>MSDMNNPSDENTGALDDLWADALNEQKATTTKSAADAVFQQLGGGDVSGAMQDIDLIMDIPVKLTVELGRTRMTIKELLRLTQGSVVALDGLAGEPLDILINGYLIAQGEVVVVADKYGVRITDIITPSERMRRLSR[9x];>[3x]MSATASTATQPKPLEWLNRLRANPRIPLIVAGSAAVAIVVAMVLWAKTPDYRTLFSNLSDQDGGAIVAQLTQMNIPYRFANGSGAIEVPADKVHELRLRLAQQGLPKGGAVGFELLDQEKFGISQFSEQVNYQRALEGELARTIETLGPVKSARVHLAMPKPSLFVREQKSPSASVTVTLEPGRALDEGQISAVVHLVSSAVAGLPPGNVTLVDQSGHLLTQSNTSGRDLNDAQLKFANDVESRIQRRIEAILSPIVGNGNVHAQVTAQLDFANKEQTEEHYSPNGDASKATLRSRQLNISEQVGAGYPGGVPGALSNQPAPPNEAPIATPPTNQQNAQNTPQTSTSTNSNSAGPRSTQRNETSNYEVDRTIRHTKMNVGDIERLSVAVVVNYKTLADGKPLPLTADQMKQIEDLTREAMGFSDKRGDTLNVVNSPFSAVDNTGGELPFWQQQSFIDQLLAAGRWLLVLVVAWILWRKAVRPQLTRRVEEAKAAQEQAQVRQETEEAVEVRLSKDEQLQQRRANQRLGAEVMSQRIREMSDNDPRVVALVIRQWMSNDHE;>MGDSILSQAEIDALLNGDSDTKDEPTPGIASDSDIRPYDPNTQRRVVRERLQALEIINERFARQFRMGLFNLLRRSPDITVGAIRIQPYHEFARNLPVPTNLNLIHLKPLRGTGLVVFSPSLVFIAVDNLFGGDGRFPTKVEGREFTHTEQRVINRMLKLALEGYSDAWKAINPLEVEYVRSEMQVKFTNITTSPNDIVVNTPFHVEIGNLTGEFNICLPFSMIEPLRELLVNPPLENSRHEDQNWRDNLVRQVQHSELELVANFADIPLRLSQILKLKPGDVLPIEKPDRIIAHVDGVPVLTSQYGTVNGQYALRVEHLINP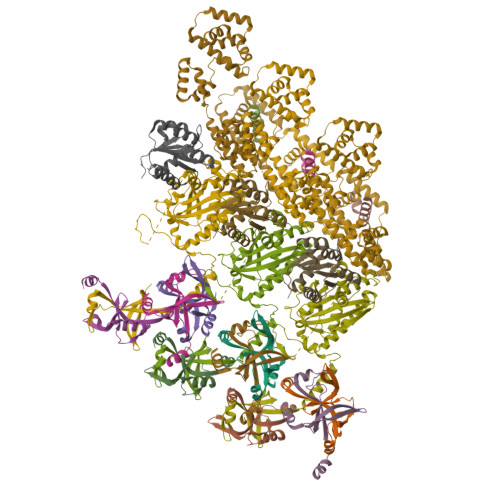ILNSLNEEQPK[3x];>MSNLSGTDKSVILLMTIGEDRAAEVFKHLSTREVQALSTAMANVRQISNKQLTDVLSEFEQEAEQFAALNINANEYLRSVLVKALGEERASSLLEDILETRDTTSGIETLNFMEPQSAADLIRDEHPQIIATILVHLKRSQAADILALFDERLRHDVMLRIATFGGVQPAALAELTEVLNGLLDGQNLKRSKMGGVRTAAEIINLMKTQQEEAVITAVREFDGELAQKIIDEMFLFENLVDVDDRSIQRLLQEVDSESLLIALKGAEPPLREKFLRNMSQRAADILRDDLANRGPVRLSQVENEQKAILLIVRRLAETGEMVIGSGEDTYV[3x];>MADKELKFLVVDKFSTMRRIVRNLLKELGFNNVEEAEDGVDALNKLQAGGFGFIISDWNMPNMDGLELLKTIRADSAMSALPVLMVTAEAKKENIIAAAQAGASGWVVKPFTAATLEEKLNKIFEKLGM[3x]>[2x]RQRWTALTPEETLFIYTRCQEEHLPADNNSRKTYIENWHQWKLQPNDHVTQCYTKCVLEGLELYDGKQK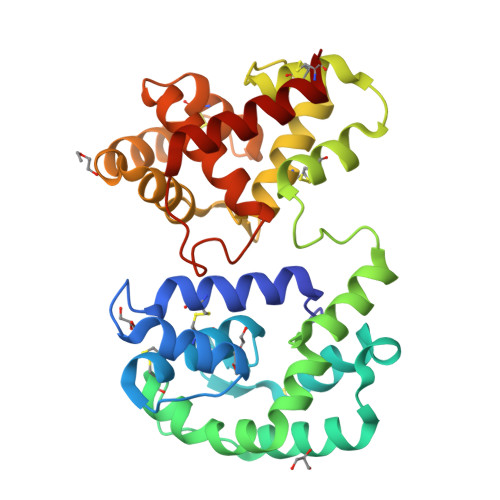KFRPGRVSSQHVAYQFLNGATADEVAKYKGAIDALEPASDSCEDLYMAYFPVHETFVNVTRKLYHGTVEGAARVYNSDPNLKRKNESLFTYCEKHVYGDQNREDMCRGRRYELTGSDELRNMIECVFRGLRYIKHGDINIDEIVRDFDHINRGDLEPRVRTILSDCRGIQPYDYYSCLINSDIREEFKLAFDYRDVRSADYAYIVKGNTYDAQKVIAEMNKVEKHVCG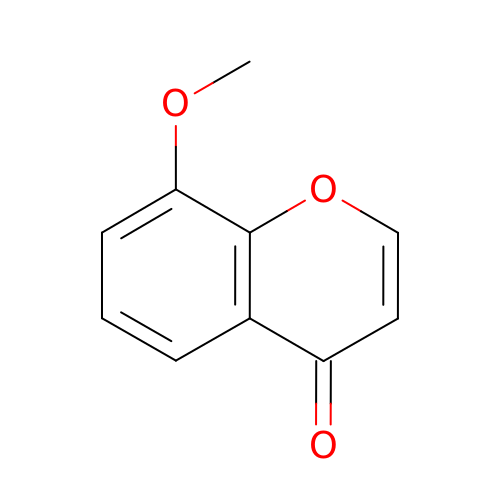8-methoxychromen-4-one | C10 H8 O3 | VLJQPDYLWJQNII-UHFFFAOYSA-N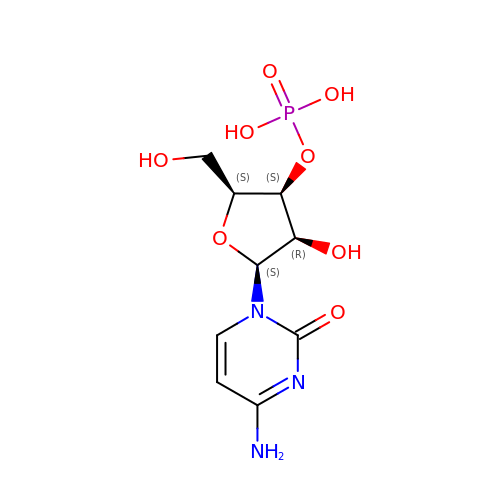[(2S,3S,4R,5S)-5-(4-amino-2-oxo-pyrimidin-1-yl)-4-hydroxy-2-(hydroxymethyl)oxolan-3-yl] dihydrogen phosphate | C9 H14 N3 O8 P | UOOOPKANIPLQPU-IHBLQFBFSA-N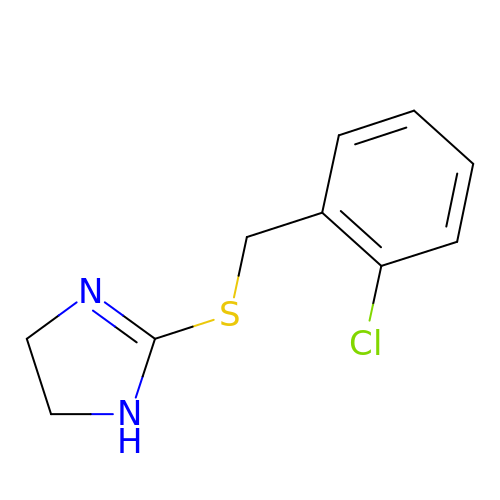2-((2-chlorobenzyl)thio)-4,5-dihydro-1H-imidazole | C10 H11 Cl N2 S | MRKZZXDCOQKXGF-UHFFFAOYSA-N> MGKKITILLGALLPFTSAVADEPALSPEAITSAQVFSTQSKETYTYVRCWYRTGNSHDESATDWEWAENPDGSYFTIDGYWWSSVRLKNMFYTNTS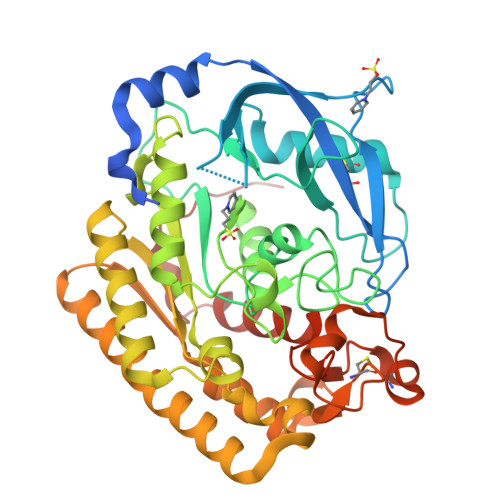QNVIKQRCEETLGVTHDAADITYFAADNRWSYNHTIWTNDPVMQADQINKIVAFGDSLSDTGNIFNAAQWRFPNPDTWFLGHFSNGFVWTEYIAQAKKLPLYNWAVGGAAGSNQYVALTGVKDQVLSYLTYAKMAKNYKPENTLFTLEFGLNDFMNYNREVVDVKTDFSTALIKLTDAGAKNIMLMTLPDATKAPQFKYSTQAEIEKVRAKIVEFNEFIKAQAAFYIIQGYNITLYDTHGLFEQLTQNPQQHGFVNASDACLNINRASSADYLYSHSLTNECATHSSDKYVFWGVTHPTTAVHKYIAEKMLAPGAGMQRFNFHHHHHH> MDQGEFIQDDNDQDYDQQEGDDENNDYMEDPQQDNNYNQNGDNLDDQGQDDDGGQNNLQQPSVPPEDDEDDDDDFPEYANEQNKRLNEIIKKKRKLIKDISAKIEEKSDRTKVLQEHLKNVEQELLHTQALIDAKNKEIETEDHMKQIAERQSGRIQSELKILEKRSIEQQEKLNDVQNQIFRGNEKMDQYKLEMNWNQEELEQWALAARQKEEDNLTLEKYKRADEVKIKELNLAIEKLTAEVGRKQNELEKEITETQAAQIELDKTAEEFKRQHEERHKLFLQWQEVTEIISKRDLAIREEGENFARIKIEIKSNKDALEERKRILKEAKEENKRIQMANELMERQNIQQISDNKHIEEQLAEKKADVEILKNQVSAFASDLSSKKNRIAILSQELLAKKQRLNAAQKKYQAHQVKLKNEEIMAKQYENDRSYAEEKYRKNEKEKKELEKEIRTQKENLFKHTQELFKHREREANLYGEIQGNMAACRNLQSHITKLNQEFQRQQELLYNAEYQIQLMERRVARAKGERTLEEKKDLENEIMNAERELGGVTGQNKELIESLKNLDDEIRTVKKKLAYVEEENTKYSSLIEELILENDMTYQDLNKIIKQKEEVLVQHDTMKLEIKKINESLNGATEKVFNLENQIYQLEMSMQEREKEIEVHKDVLMTEHKAAEEERHKIAVELAERKNKVKNLKIKYESLVQKNKASNGEVESVHEHSQAYYVIKAAQEREELQRKGDELNAKILKNEKELKALDNTLNHLKNRNSNYRDKFLNKGVTTQHREEAEGLEEQCRAASQNLFKKRDELQKLQKEQEEDTRRYTEIKNKL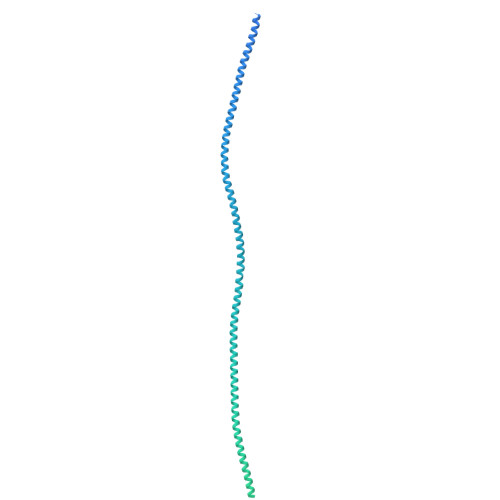ERLYEQHQSLDQEISKYQKDIDQQGDKLQRAQNSLQRNYQLAVNKNQNFINPKNPHMIQVKLDNQNNLYKTLLQGLYSLQQDIPELSSVVDEILKEQRIQNNKAPSSIDINSKRSSQSGRSQRSQRSNISNQ> MGQDPVELAMFGLRHMEPDLS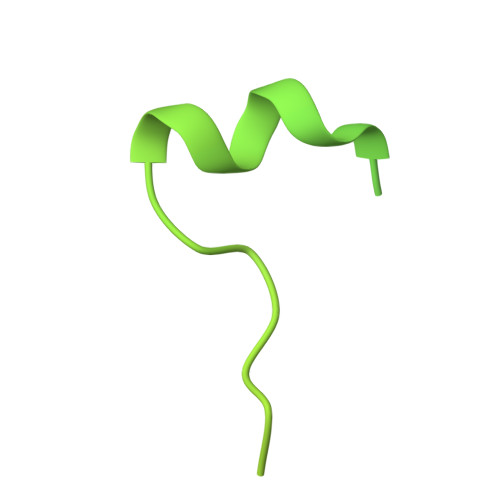ARVTIYQVPLPKDSTGAADPPQPHIVGIQSPDQQAALARHNPARPVFVEGPFSLWLRNKCVYYHILRADLLPPEEREVEETPEEWNLYYPMQLDLEYVRSGWDNYEFDINEVEEGPVFAMCMAGAHDQATMAKWIQGLQETNPTLAQIPVVFRLAGSTRELQTSSAGLEEPPLPEDHQEEDDNLQRQQQGQSLEHHHHHH> TPTTFVHLFEWNWQDVAQECEQYLGPKGYAAVQVSPPNEHITGSQWWTRYQPVSYELQSRGGNRAQFIDMVNRCSAAGVDIYVDTLINHMAAGSGTGTAGNSFGNKSFPIYSPQDFHESCTINNSDYGNDRYRVQNCELVGLADLDTASNYVQNTIAAYINDLQAIGVKGFRFDASKHVAASDIQSLMAKVNGSPVVFQEVIDQGGEAVGASEYLSTGLVTEFKYSTELGNTFRNGSLAWLSNFGEGWGFMPSSSAVVFVDNHDNQRGHGGAGNVITFEDGRLYDLANVFMLAYPYGYPKVMSSYDFHGDTDAGGPNVPVHNNG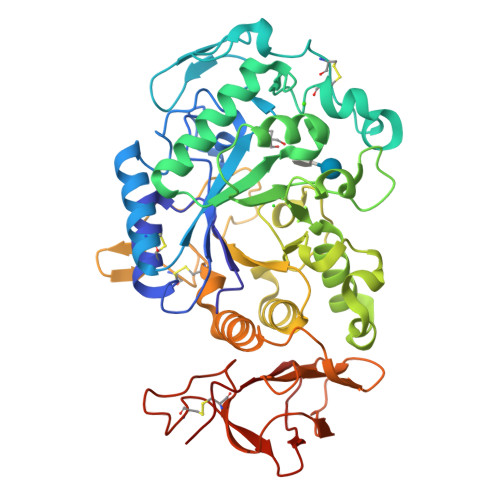NLECFASNWKCEHRWSYIAGGVDFRNNTADNWAVTNWWDNTNNQISFGRGSSGHMAINKEDSTLTATVQTDMASGQYCNVLKGELSADAKSCSGEVITVNSDGTINLNIGAWDAMAIHKNAKLN>MTSPAKFKKDKEIIAEYDTQVKEIRAQLTEQMKCLDQQCELRVQLLQDLQDFFRKKAEIEMDYSRNLEKLAERFLAKTRSTKDQQFKKDQNVLSPVNCWNLLLNQVKRESRDHTTLSDIYLNNIIPRFVQVSEDSGRLFKKSKEVGQQLQDDLMKVLNELYSVMKTYHMYNADSISAQSKLKEAEKQEEKQIGKSVKQEDRQTPRSPDSTANVRIEEKHVRRSSVKKIEKMKEKRQAKYTENKLKAIKARNEYLLALEATNASVFKYYIHDLSDLIDQCCDLGYHASLNRALRTFLSAELNLEQSKHEGLDAIENAVENLDATSDKQRLMEMYNNVFCPPMKFEFQPHMGDMASQLCAQQPVQSELVQRCQQLQSRLSTLKIENEEVKKTMEATLQ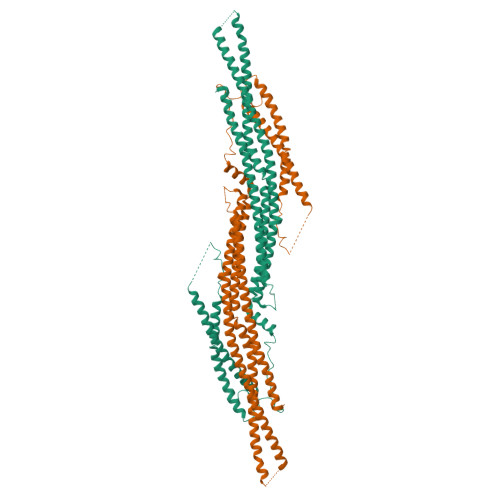TIQDIVTVEDFDVSDCFQYSNSMESVKSTVSETFMSKPSIAKRRANQQETEQFYFTKMKEYLEGRNLITKLQAKHDLLQKTLGESQRT[2x]>[2x]GSHMASKPIEDYGKGKGRIEPMYIPDNTFYNADDFLVPPHCKPYIDKILLPGG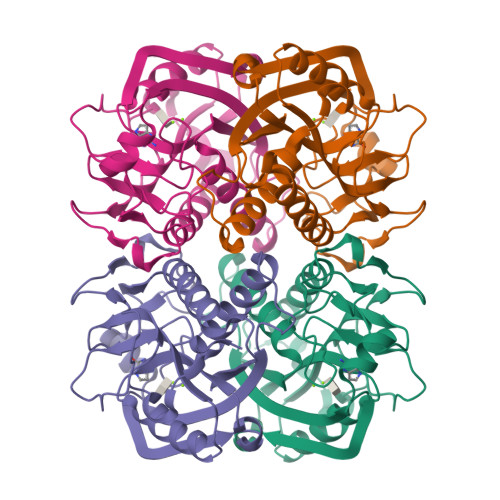LVKDRVEKLAYDIHRTYFGEELHIICILKGSRGFFNLLIDYLATIQKYSGRESSVPPFFEHYVRLKSYQNDNSTGQLTVLSDDLSIFRDKHVLIVEDIVDTGFTLTEFGERLKAVGPKSMRIATLVEKRTDRSNSLKGDFVGFSIEDVWIVGCCYDFNEMFRDFDHVAVLSDAARKKFEK all-trans okenone | C41 H54 O2 | 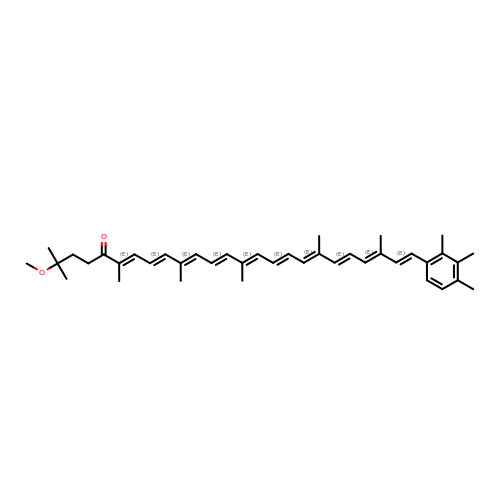FSQZIFSGNDUYRQ-TYKRLFMMSA-N> GPGSEFSEAISIDLLQKKGLVKAVNIAVDLIVAHFGTSRDPGVKAKLGNSSVSPNVGHLVLKYLCPAVRAVLEDGLKAFVLDVIIGQRKNMPWSVVEASTQLGPSTKVLHGLYNKVSQFPELTSHTMRFNAFILGLLNIRSLEFWFNHLYNHEDIIQTHYQPWGFLSAAHTVCPGLFEELLLLLQPLALLPFS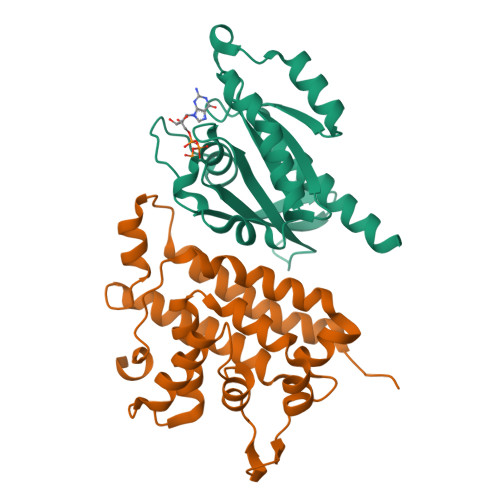LDLLFQHRLLQS;> GPGSEFMARDYDHLFKLLIIGDSGVGKSSLLLRFADNTFSGSYITTIGVDFKIRTVEINGEKVKLQIWDTAGLERFRTITSTYYRGTHGVIVVYDVTSAESFVNVKRWLHEINQNCDDVCRILVGNKNDDPERKVVETEDAYKFAGQMGIQLFETSAKENVNVEEMFNCITELVLRAKKDNLAKQQ> GS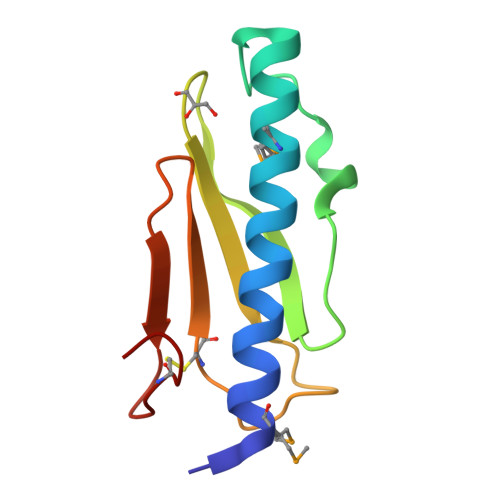HMRRVRLSEVRTTLLHNAQTMERYYRQKGTFKTYDKNKLKQNKYFNVTLSKVSPDHFTLQADPNPTTNDGETCVVTLNDGGTIAASGTNQSCPGFD> MRIDGHRQVVSN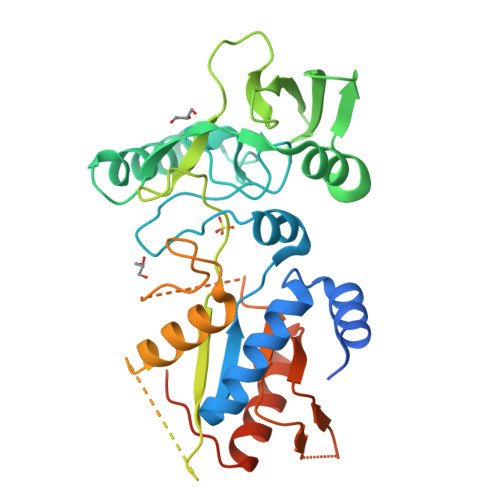ATAQPGPLLRPADMQARALQDLFDAQGVGVPVEHALRMQAVARQTNTVFGIRPVERIVTTLIEEGFPTKGFSVKGKSSNWGPQAGFICVDQHLSKREDRDTAEIRKLNLAVAKGMDGGAYTQTDLRISRQRLAELVRNFGLVADGVGPVRLLTAQGPSGKRYEFEARQEPDGLYRISRLGRSEAVQVLASPACGLAMTADYDLFLVAPSIEAHGSGGLDARRNTAVRYTPLGAKDPLSEDGFYGREDMARGNITPRTRQLVDALNDCLGRGEHREMFHHSDDAGNPGSHMGDNFPATFYLPRAMEHRVGEESVRFDEVCVVADRKSFSLLVECIKGNGYHFTAHPDWNVPLRPSFQEALDFFQRKV The COMMD (Copper Metabolism Murr1 (Mouse U2af1-rs1 region 1) Domain) proteins are highly conserved in metazoans and unicellular protozoa. There are ten family members that play key roles in intracellular trafficking and in the regulation of transcription. A hallmark of the COMMD family members is a highly conserved C-terminal sequence of ~70–80 amino acids called the COMM domain, which has no known structure. The N-terminal domain of these proteins, which we refer to as the HN (helical N-terminal) domain, is more variable in sequence across the ten proteins, and is proposed to ascribe unique functions to the different family members.

Overall, the Commd9 N-terminal domain has a globular architecture and is composed of a six-helix bundle with a meander topology. We therefore refer to this domain as the HN (Helical N-terminal) domain. The overall structure of the HN domain has a similar all α-helical fold to the equivalent domain of Commd1, which was previously determined by NMR. Compared to Commd1 however, the HN domain of Commd9 has an additional α-helix at its N-terminus that packs down on top of the structure, and a large disordered loop in Commd1 is better resolved in Commd9. In Commd9 the α4 helix forms a central core element that extends the length of the HN domain. The electrostatic surface of the Commd9 HN domain reveals the presence of two basic patches and a negatively charged region, but it is not clear yet what their functional significance might be. Mapping sequence conservation of the Commd9 HN domain across species shows conserved surface residues mainly in the α1 helix region. Bioinformatics and secondary structure analyses of the human COMMD proteins however, shows that in all of the family members the HN domain is very likely to share the same α-helical topology, as well as across various species of Commd9. Our biophysical, structural and bioinformatics analyses however show that the HN domain is a structurally conserved feature shared by all COMMD family members.

>MSGAMAALTAEHFAALQSLLKASSKDVVRQLCQESFSSSALGLKKLLDVTCSSLSVTQEEAEELLQALHRMTRLVAFRDLSSAEAILALFPENFHQNLKNLLTKIMLEHVSTWRTEAQANQ[6x]> MENTENSVASKSIKNLEPKIIHGSESMASGISLDNSYKMDYPEMGLCIIINNKNFHKSTGMTSRSGTDVDAANLRETFRNLKYEVRNKNDLTREEIVELMRDVSKEDHSKRSSFVCVLLSHGEEGIIFGTNGPVDLKKITNFFRGDRCRDLTGKPKLFIIQACRG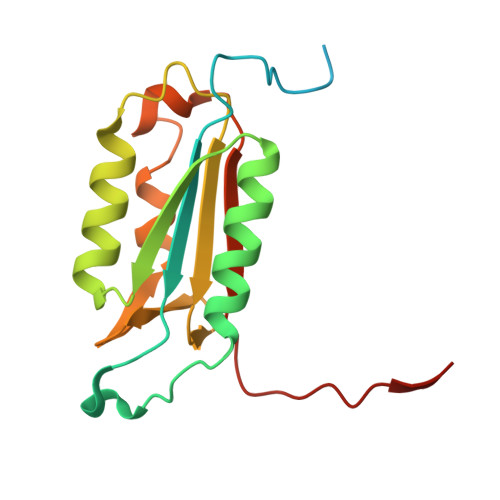TELDCGIETD> KLGKLQYSLDYDFQNNQLLVGIIQAAELPALDMGGTSDPYVKVFLLPDKKKKFETKVHRKTLNPVFNEQFTFKVPYSELGGKTLVMAVYDFDRFSKHDIIGEFKVPMNTVDFGHVTEEWRDLQSAEKEEQEKLGDICFSLRYVPTAGKLTVVILEAK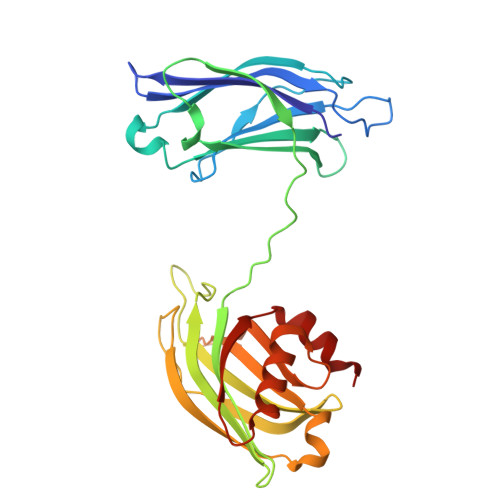NLKKMDVGGLSDPYVKIHLMQNGKRLKKKKTTIKKNTLNPYYNESFSFEVPFEQIQKVQVVVTVLDYDKIGKNDAIGKVFVGYNSTGAELRHWSDMLANPRRPIAQWHTLQVEEEVDAMLAVKK1,4-DIDEOXY-1,4-[[2S,3S)-2,4-DIHYDROXY-3-(SULFOXY)BUTYL]EPISELENONIUMYLIDENE]-D-ARABINITOL 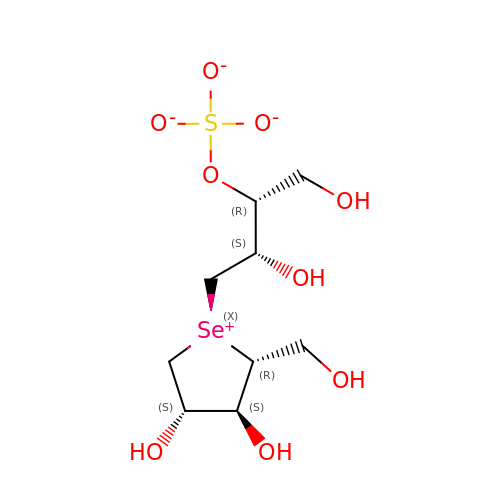INNER SALT | C9 H18 O9 S Se | WLNWUNIGATZIKW-ZCYZNMBRSA-L> NCKVKDEQKSRALTIIVFGASGDLAKKKTFPALFDLYCGGLLPPEVNIIGYARTKVDDVEKWKHETLMKYFSNLSERGCHAEDFLKHISYFCGAYDSVDDFKRLDAVIREKENAFKGPEKGGNRLFYLALPPSVFASVCESIHKGAMPQEVGGWVRVIIEKPFGRDTKSSAELSQALEPFFDESQLYRIDHYLGKEMVQNIITTRFANRIFSAVWNASNIACVQITFKETIGTEGRGGYFDNIGIIRDVMQNHLTQILALLAMEKPRSLDAECIRDEKVSVLKCIEPITKENCVLGQYTASADGSIPGYLEDVTVPEGSTCPTFAVMRLNINNDRWAGVPFILKAGKAVEQKYVAIRIQFRDEVH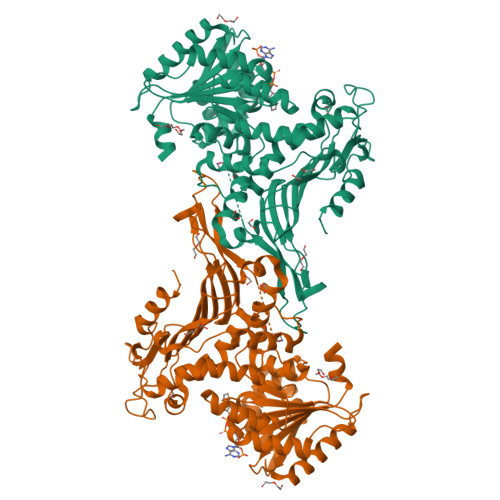PYGEATQRNELVIRAQPSEAMYVKITTKVPGLSGDLRQTHQTELDLTYHTRYDVRLPDAYESLINDALLGNSTNFVRKDELDVAWRIFTPLLHQIDSGEIKPIPYQAGTRGPKEADEFIANNGFKHQKGYHWLPSNKL> MAGARQELDTFTRGLKGLDGQFSQRVTDANGRVKENSSGRVALATPRQFRWEYAKPYKQLIVADGKKVWVFDPDLEQVTVRAQGSEEQNSPLVALIDPTRLDKQYDVSEEAAPRDGLQWLSLTPKVDTDASFQMASLGFGKDGLAKMEVVDAV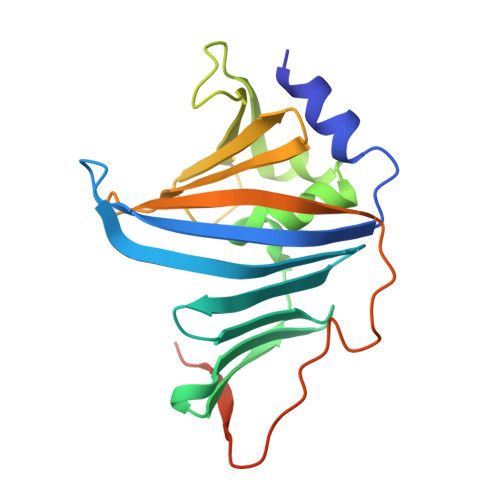GQRTAISFSGWKRNPAFAADTFRYTPGKGVDVVGDAQAENLYFQSHHHHHH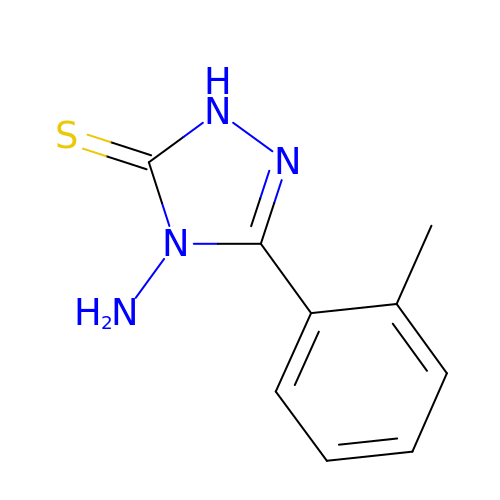4-AMINO-5-(2-METHYLPHENYL)-2,4-DIHYDRO-3H-1,2,4-TRIAZOLE-3-THIONE | C9 H10 N4 S | CUEYNOAJNUCBAP-UHFFFAOYSA-N>MAEYVFSDAPKDSHGNGVKDAVPGKQPEELPPAPRYFQGENTAGFMRPVRFEGDITNLEVVGEIPKSIEGTFYRVMPEPHLPSFIPNDPWFNGDGNISGFYFKDGHVDLKQRYVRTEKFVREAEARRSLLGKYRNRYTDLVEFKIRSTANGNIVYWRGQLLALKEDSPPYAMDPETLETFGVYDFDGQLPSLTFTAHPKFDPVTREMVCFGYEAKGDGTRDICYYSFGPDGKIAETVWLVSPVCGMIHDFAVTENFVIFPIIPLVCDVERMKQGGDHWQWDYSIPMYIGVLPRRGAQGSDVKWFEAPHGFAGHVANAFEDDKGHIQLQMAYAKDNVFFWWPDANGKGPRPGEVEAHFANFVLDYQSDKLPLAEPTYLVDDDMEFPRIDDRVATRKHKHTFFCIFDRKPGVTDFEFVMPRAGGGAPMSNGLAHLNHETGDIQRYLPGPRKLTGECIFIPRNSEAAEGDGYVMVLLANYEDMCSELAVLDTKDLTNEVALIKLPVRLRPGLHGNWVDKSDVDGHPAPL[4x]

Carotenoid cleavage dioxygenases (CCDs) are non-heme FeII enzymes that catalyze the oxidative cleavage of alkene bonds in carotenoids, stilbenoids, and related compounds. pmcCarotenoid cleavage dioxygenases (CCDs) are a broadly distributed superfamily of enzymes that catalyze the reaction of dioxygen (O2) with carotenoids, stilbenoids, and related redox-active polyenes. These enzymes use a mononuclear non-heme FeII center to activate O2 for reaction with a specific alkene group in the substrate, generating carbonyl-containing products of importance in biological processes such as hormonal signaling and light detection. Unlike many mononuclear non-heme iron dioxygenases that coordinate their FeII centers using a 2-His, 1-Glu/Asp “facial triad” motif, CCDs use a 4-His cluster, three of which hydrogen bond to second-sphere carboxylates (Glu/Asp). While one coordination position is occupied by a solvent ligand as demonstrated by several crystallographic and spectroscopic investigations, the other is vacant because of apparent occlusion by a nearby methyl group of a semiconserved, second sphere residue (i.e., Thr/Val/Ile), making CCDs five-coordinate (5C) in their resting FeII states.

To investigate whether reduction in side-chain volume would allow solvent binding at the sixth position, site-directed mutagenesis was used to introduce a T151G substitution in CAO1, thereby opening the maximal potential space for ligand coordination. Crystallography on the T151G FeII–CAO1 piceatannol complex showed a piceatannol binding conformation in T151G FeII–CAO1 resembling that observed for the wildtype enzyme, the main difference being a ∼10° rotation of the β-ring toward the vacancy left from the absent Thr side chain. Two solvent molecules remained bound to the iron center trans to His197 and His313. Notably the iron-solvent bond lengths were shortened by ∼0.4 to 0.5 Å in the ES complex as compared with the resting T151G FeII–CAO1 structure. However, the resolution of the diffraction data was insufficient to allow modeling of the mixture of 5C and 6C species found by MCD spectroscopy. The energies and intensity patterns of these four transitions are consistent with one 6C and one 5C species, constituting ∼85% and ∼15% of the sample, respectively, as estimated by comparison of the intensities at 11,500 cm-1. These data indicate that substrate binding leads to dissociation of one iron-bound water in a subset of the molecules in the sample. We find that while the resting FeII site in the less constrained T151G CAO1 variant is 6C, substrate binding induces loss of a water ligand in a fraction of sample, which appears to confer higher binding affinity for NO.> XSKGDPGPPG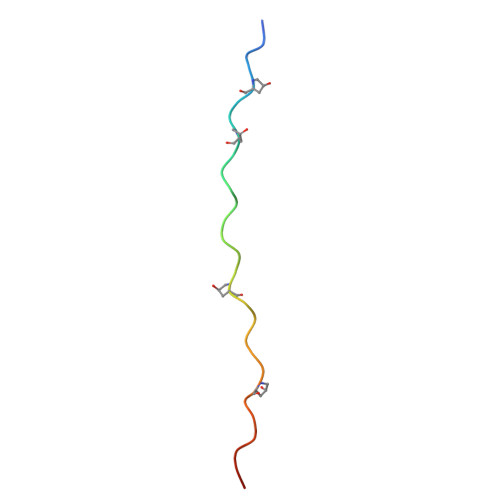DRGPKGPPGYKGPPGDKGFRGX> PVQLNLLYVQARDDILNGSHPVSFDKACEFAGYQCQIQFGPHNEQKHKPGFLELKDFLPKEYIKQKGERKIFMAHKNCGNMSEIEAKVRYVKLARSLKTYGVSFFLVKEKMKGKNKLVPRLLGITKECVMRV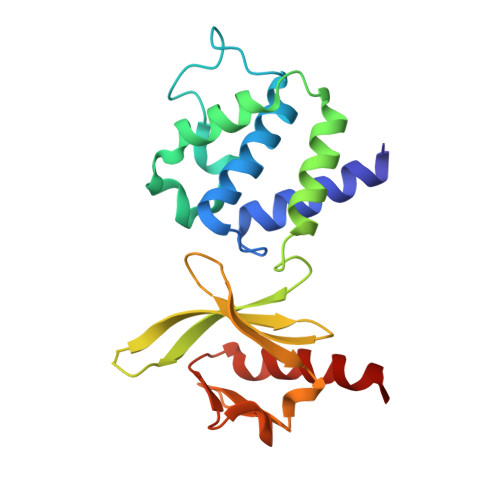DEKTKEVIQEWSLTNIKRWAASPKSFTLDFGDYQDGYYSVQTTEGEQIAQLIAGYIDIIL> MGSDKIHHHHHHMAYLEVLRYLYHKRPMGKVKPGLERISMLLSKLGNPHLEYKTIHIGGTNGKGSVANMVSNILVSQGYRVGSYYSPHLSTFRERIRLNEEYISEEDVVKIYETMEPILNELDKEE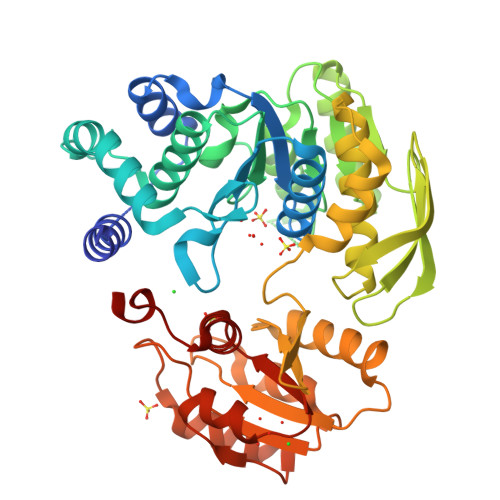IFSPSFFEVVTAMAFLYFAEKNVDIAVLEVGLGGRLDATNVVFPLCSTIVTVDRDHEKTLGYTIEQIAWEKSGIIKERVPLVTGERKREALKVMEDVARKKSSRMYVIDKDFSVKVKSLKLHENRFDYCGENTFEDLVLTMNGPHQIENAGVALKTLEATGLPLSEKAIREGLKNAKNLGRFEILEKNGKMYILDGAHNPHGAESLVRSLKLYFNGEPLSLVIGILDDKNREDILRKYTGIFERVIVTRVPSPRMKDMNSLVDMAKKFFKNVEVIEDPLEAIESTERATVVTGSLFLVGYVREFLTTGKINEEWKL> GPHMGNIMSASFA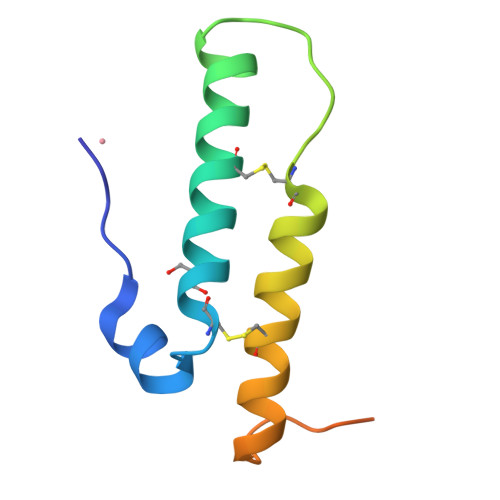PECTDLKTKYDSCFNEWYSEKFLKGKSVENECSKQWYAYTTCVNAALVKQGIKPALDEAREEAPFENGGKL> MDIRPNHT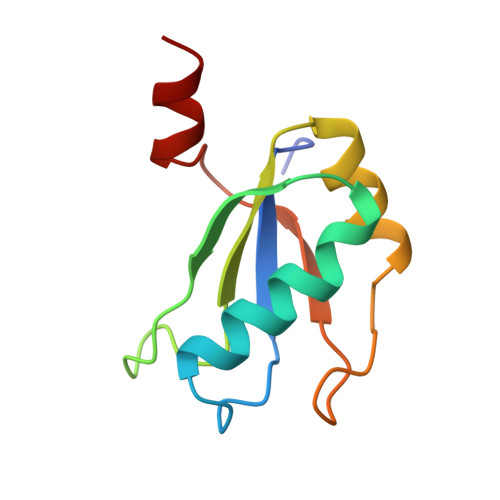IYINNMNDKIKKEELKRSLYALFSQFGHVVDIVALKTMKMRGQAFVIFKELGSSTNALRQLQGFPFYGKPMRIQYAKTDSDIISKMRG>MIVIFVDFDYFFAQVEEVLNPQYKGK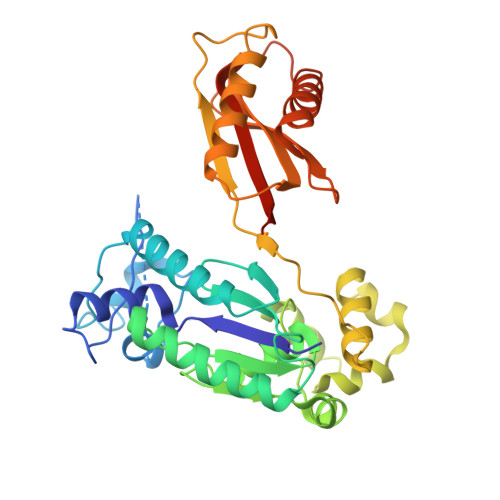PLVVSVYSGRTKTSGAVATANYEARKLGVKAGMPIIKAMQIAPSAIYVPMRKPIYEAFSNRIMNLLNKHADKIEVASIDEAYLDVTNKVEGNFENGIELARKIKQEILEKEKITVTVGVAPNKILAKIIADKSKPNGLGVIRPTEVQDFLNELDIDEIPGIGSVLARRLNELGIQKLRDILSKNYNELEKITGKAKALYLLKLAQNKYSEPVENKSKIPHGRYLTLPYNTRDVKVILPYLKKAINEAYNKVNGIPMRITVIAIMEDLDILSKGKKFKHGISIDNAYKVAEDLLRELLVRDKRRNVRRIGVKLDNIIINKTNLSDFFDI[2x]Invertebrates possess a different gap junction protein family, termed innexins, that is essential for eating and developmental functions in Caenorhabditis elegans and for electrical synapses in Drosophila7. We recently revealed that the C. elegans innexin-6 (INX-6) gap junction channel structure is a 16-subunit oligomer, that is, a hexadecamer, with larger dimensions than those of connexins. Here we report the atomic resolution structures of INX-6 determined by cryo-EM in combination with GraDeR.

To construct a full gap junction channel of INX-6, particles showing the properties of docked junction channels were picked from the same set of cryo images. The density map of the INX-6 gap junction channel was reconstructed at 3.6 Å resolution from 35,608 particles with D8 symmetry. A model of the INX-6 gap junction channel was refined after fitting the atomic model of the INX-6 hemichannel into the density map of the INX-6 gap junction channel. The hexadecameric structure of the INX-6 gap junction channel appears similar to the Cx26 structure, a tsuzumi-shape. The channel height is estimated to be about 200 Å, which is smaller than that observed in INX-6ΔN15. The extracellular docking surface of a hemichannel provides cavities to accommodate the E2 β-hairpins from the opposing hemichannel, which is reminiscent of a model previously proposed for connexin24. The inner and outer lobes of E1 straddle the E2 β-hairpin stacks whereby the E2 β-hairpins serve as a wall to prevent from leakage of permeates to the extracellular space. The pore pathway has a high positive potential and is constricted at two sites for each hemichannel (four per junction channel). The narrowest constrictions are provided by the N-termini making a funnel configuration with an 18-Å diameter (Fig. 4b—membrane and Fig. 5a), and others are given by E1Hs (Fig. 4b—extracellular and Fig. 5a).

>MASQVGAINSVNALISRVFVQPKGDLADRLNSRVTVVILAVSSALLLSSHFIGDPITCWTPAQFNAQWVNFVNQYCFVHGTYFVPLDQQLAFEEEERTKVSIQYYQWVPYVFALQAFLFYIPRFIWKAMIAYSGYDLAAAVKYVDRFWSENRDKDDKFKTRLAAFEGRPSVYIWDGIRLARKKRSRNMALFYTLSTVWQAVNAWIQFYILTQLLDSSIYTLWGPSILGDLLQGNDWQTTGHFPRIVHCDFNRRRPASVQLDTVLCVLTLNIYYEKLFIFLWFWLVFVAVVSTVNCFKWIYYLCNKTKAQKTIKNYLSTAPIKSTISDDQFFSALGEDGLFIMDQMALNLGDIPASYLTISMRNICQDFIESEDYIDEERTPFVKSIKHT[16x]{5-[(2E)-2-methyl-3-phenylprop-2-en-1-ylidene]-4-oxo-2-thioxo-1,3-thiazolidin-3-yl}acetic acid | C15 H13 N O3 S2 | 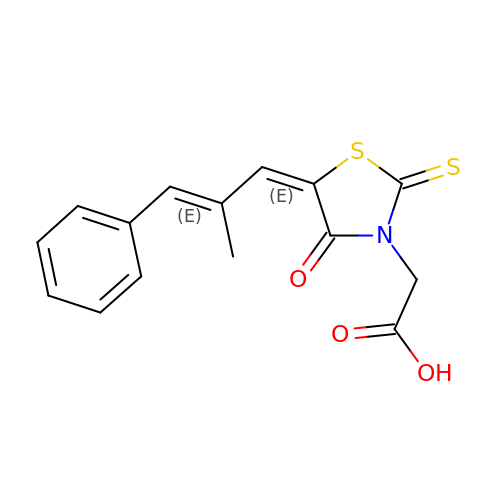CHNUOJQWGUIOLD-KEBJEMEDSA-N>[2x]MATTTSNMFLYSLTIQPPTTITQALLGQFSGTKEQQIITASGSRLTLLQPDPRQGKVNTIVSHDIFGIIRAMAAFRLAGSHKDYIILATDSGRIAIIEYLPKENRFQRIHLETFGKSGVRRVIPGQYLAADPKGRACLIASVEKN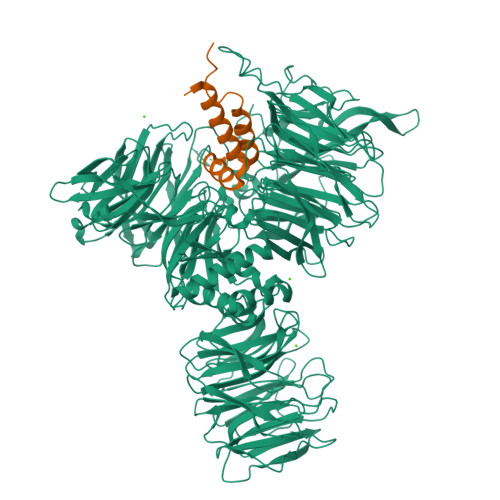KLVYVLNRNAQAELTISSPLEAHKPGVIVLSLVALDVGYSNPVFAALEYEYSEADQDPTGQAAKQLEMQLVYYELDLGLNHVVRKWSDTVDPTSSLLFQVPGGNDGPSGVLVCGEENITYRHSNQEAFRVPIPRRRGATEDPNRKRTIVAGVMHKLKGSAGAFFFLLQTEDGDLFKVTIDMVEDEKGNPTGEVKRVKIKYFDTVPIAHSLCILKSGFLFVASEFGNHHFYQFEKLGDDDDEPEFTSDDFPADWNAPYNPVYFKPRPLENLVLVESIDSMNPLVGCKVANLTGEDAPQIYAICGNGARSSFRMLKHGLEVSEIVASELPGTPSAVWTTKLTKYDEYDAYIVLSFTNATLVLSIGETVEEVSDSGFLTTVPTLAVQQMGEEGLIQIHPKGIRHIVQGRVNEWPAPQHRSIVAATTNENQVVIALSSGEIVYFEMDADGSLAEYDEKKQMSGTVTSLSLGKVPEGLRRSSFLAVGCDDCTVRILSLDPESTLEMKSIQALTAAPSSLLIMSMEDSTGGTTLYLHIGLHSGVYLRTVLDEITGELTDTRQKFLGPKPTKLFQVTVQNQTCVLALSSRPWLGYTAPITRNFVMTPLSYTELGYTWSFNSEQCQEGMVGIHANYLRIFTIEKLGQTMIQKSCPLTYTPKRLVKHPEQPYFYVIEADNNTLPPELRAQLLEQSGAVNGDATVLPPEDFGYPKARGRWASCIEIVDPVSEEQPRVLKRIELEGNEAAVSAAVVPFASQDGESFLIVGTGKDMVLNPRASTEGAIHVYRFIDDGRDLEFIHKTIIEEPPLAFCPFQGRLLAGIGKMLRIYDLGLKQLLRKAQAEVSPQLIVSLDTRHNRIVVGDVQHGMTYVVYKPDSNKLIPFADDTIARWTTCTTMVDYESVAGGDKFGNLWIVRCPERASLESDEPGSEVQLLHARPYLHGAPNRLDLMAHFYPQDLPTSICKTNLVVGGQDVLVWSGIQGTVGVLIPFVTREDADFFQNLESHMRAEDPPLAGRDHLIYRGYYVPVKGVIDGDLCERFTLLPNDKKQMIAGELDRSVREIERKISDIRTRSAF;>MADKLRNQQELERLQAKYVGTGHPDTTSWEWKTNIHRDTYSSIVGHPPLLSYMALAQNEPVAKFRVQMIRKMLQPVGPPPPREEDIIMSNTQNGS[2x]MLKL is a key player in the necroptosis pathway, encompassing a C-terminal regulatory and an N-terminal executioner domain. It gets activated through phosphorylation of Thr357 and Ser358 in its pseudokinase domain by RIP3 kinase and subsequently oligomerizes via its executioner domain and inserts into the membrane. To this end, displacement of the auto-inhibitory brace helix (α-helix 6) from the four-helix bundle is required, which depends on a specific composition of phospholipids in the membrane. Currently, two classes of compounds are reported to inhibit MLKL by covalently binding to Cys86 in the short α-helix 4 located on top of the four-helix bundle, which comprises α-helices 1, 2, 3, and 5.

Here, we present the high-resolution structures of the human MLKL executioner domain in complex with a covalent inhibitor of the xanthine class solved by X-ray crystallography and in solution by NMR spectroscopy. Next, we determined the protein–ligand costructure with the newly synthesized xanthine Cpd 3. The binding pose of Cpd 3 was very similar in the NMR and the X-ray structures of the MLKL:Cpd 3 complex. Overall structural changes upon complex formation were minor, and the overall fold of MLKL was preserved. The most profound structural change induced by covalent modification of Cys86 was the alteration of the conformation of Phe148. This resulted in a stacking interaction with the aromatic ring of the xanthine core, therefore creating an additional contact between α-helix 6 and the four-helix bundle. Minor differences between the NMR and X-ray costructure were most likely due to variations in construct lengths (residues 1 to 154 in the NMR and 1 to 150 in the X-ray structure, respectively). Here, we report that the xanthine class of inhibitors acts by stabilizing the packing of α-helix 6 against the four-helix bundle through the formation of a stabilizing π–π-stacking interaction between Phe148 located in α-helix 6 and the xanthine core. Addition of 500 µM Cpd 3 shifted the population back to the auto-inhibited state of α-helix 6 (pact 19%), suggesting that the stabilization by the covalent modification protects MLKL from activation. Mutation of Phe148 to alanine leads to loss of the stabilization of the auto-inhibited state of MLKL by xanthine class compounds, confirming the key role of the observed π–π-stacking interaction for the activity of the xanthine class.

>GSPGENLKHIITLGQVIHKRCEEMKYCKKQCRRLGHRVLGLIKPLEMLQDQGKRSVPSEKLTTAMNRFKAALEEANGEIEKFSNRSNICRFLTASQDKILFKDVNRKLSDVWKELSLLLQVEQRMPVSPISQGASWAQEDQQDADEDRRAFQM[2x]>MRKKISIIGAGFVGSTTAHWLAAKELGDIVLLDIVEGVPQGKALDLYEASPIEGFDVRVTGTNNYADTANSDVIVVTSGAPRKPGMSREDLIKVNADITRACISQAAPLSPNAVIIMVNNPLDAMTYLAAEVSGFPKERVIG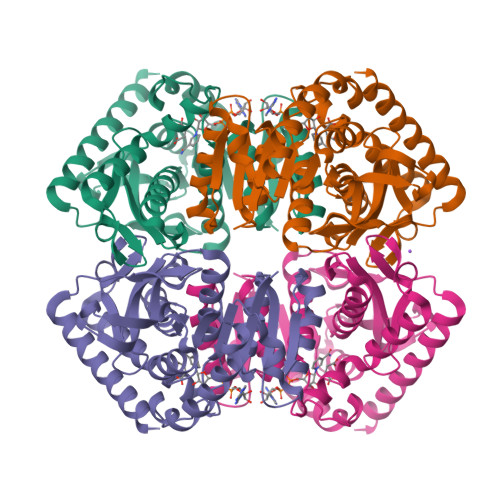QAGVLDAARYRTFIAMEAGVSVKDVQAMLMGGHGDEMVPLPRFSTISGIPVSEFIAPDRLAQIVERTRKGGGEIVNLLKTGSAYYAPAAATAQMVEAVLKDKKRVMPVAAYLTGQYGLNDIYFGVPVILGAGGVEKILELPLNEEEMALLNASAKAVRATLDTLKSL[2x]>[2x]HHPCCSNPCQNRGECMSTGFDQYKCDCTRTGFYGENCTTPEFLTRIKLLLKPTPNTVHYILTHFKGVWNIVNNIPFLRSLIMKYVLTSRSYLIDSPPTYNVHYGYKSWEAFSNLSYYTRALPPVADDCPTPMGVKGNKELPDSKEVLEKVLLRREFIPDPQGSNMMFAFFAQHFTHQFFKTDHKRGPGFTRGLGHGVDLNHIYGETLDRQHKLRLFKDGKLKYQVIGGEVYPPTVKDTQVEMIYPPHIPENLQFAVGQEVFGLVPGLMMYATIWLREHNRVCDILKQEHPEWGDEQLFQTSRLILIGETIKIVIEDYVQHLSGYHFKLKFDPELLFNQQFQYQNRIASEFNTLYHWHPLLPDTFNIEDQEYSFKQFLYNNSILLEHGLTQFVESFTRQIAGRVAGGRNVPIAVQAVAKASIDQSREMKYQSLNEYRKRFSLKPYTSFEEL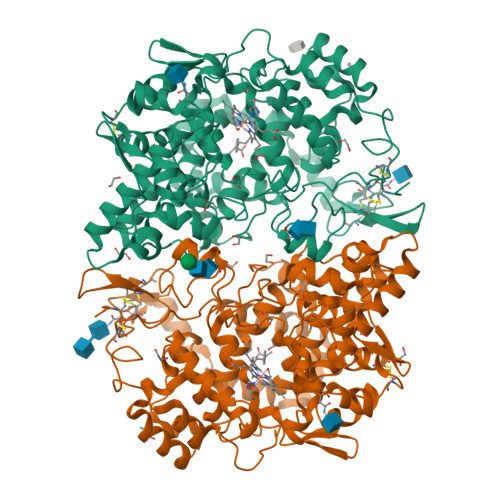TGEKEMAAELKALYSDIDVMELYPALLVEKPRPDAIFGETMVELGAPFSLKGLMGNPICSPQYWKPSTFGGEVGFKIINTASIQSLICNNVKGCPFTSFNV> GPLGSPEFMAQGTLIRVTPEQPTHAVCVLGTLTQLDICSSAPEDCTSFSINASPGVVVDIAHSPPAKK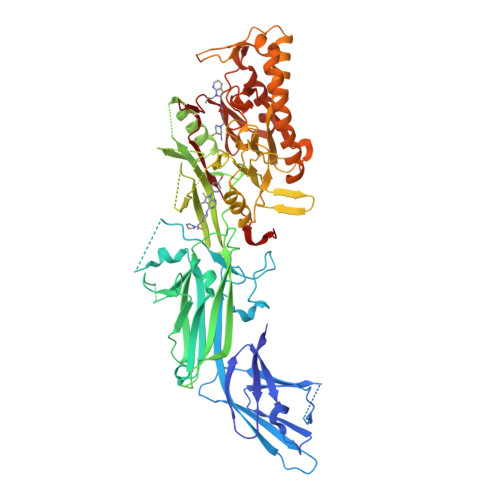KSTGSSTWPLDPGVEVTLTMKAASGSTGDQKVQISYYGPKTPPVKALLYLTAVEISLCADITRTGKVKPTRAVKDQRTWTWGPCGQGAILLVNCDRDNLESSAMDCEDDEVLDSEDLQDMSLMTLSTKTPKDFFTNHTLVLHVARSEMDKVRVFQATRGKLSSKCSVVLGPKWPSHYLMVPGGKHNMDFYVEALAFPDTDFPGLITLTISLLDTSNLELPEAVVFQDSVVFRVAPWIMTPNTQPPQEVYACSIFENEDFLKSVTTLAMKAKCKLTICPEEENMDDQWMQDEMEIGYIQAPHKTLPVVFDSPRNRGLKEFPIKRVMGPDFGYVTRGPQTGGISGLDSFGNLEVSPPVTVRGKEYPLGRILFGDSCYPSNDSRQMHQALQDFLSAQQVQAPVKLYSDWLSVGHVDEFLSFVPAPDRKGFRLLLASPRSCYKLFQEQQNEGHGEALLFEGIKKKKQQKIKNILSNKTLREHNSFVERCIDWNRELLKRELGLAESDIIDIPQLFKLKEFSKAEAFFPNMVNMLVLGKHLGIPKPFGPVINGRCCLEEKVCSLLEPLGLQCTFINDFFTYHIRHGEVHCGTNVRRKPFSFKWWNMVP>[2x]GGCG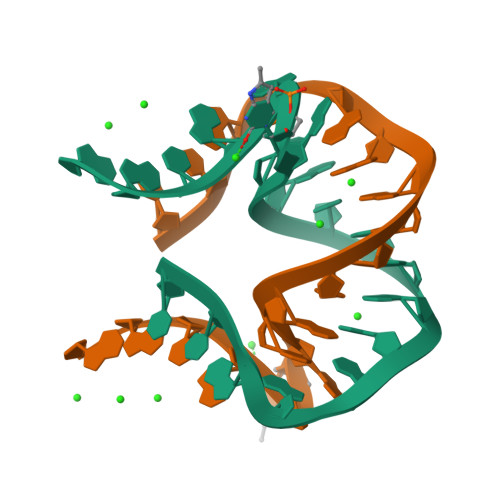ACGAACCGGGGAGCC>MTERIRNVALRSKVCPAETASELIKHGDVVGTSGFTGAGYPKEVPKALAQRMEAAHDRGEKYQISLITGASTGPQLDGELAKANGVYFRSPFNTDATMRNRINAGETEYFDNHLGQVAGRAVQGNYGKFNIALVEATAITEDGGIVPTSSVGNSQTFLNLAEKVIIEVNEWQNPMLEGIHDIWDGNVSGVPTRDIVPIVRADQRVGGPVLRVNPDKIAAIVRTNDRDRNAPFAAPDETAKAIAGYLLDFFGHEVKQNRLPPSLLPLQSGVGNVANAVLEGLKEGPFENLVGYSEVIQDGMLAMLDSGRMRIASASSFSLSPEAAEEINNRMDFFRSKIILRQQDVSNSPGIIRRLGCIAMNGMIEADIYGNVNSTRVMGSKMMNGIGGSGDFARSSYLSIFLSPSTAKGGKISAIVPMAAHVDHIMQDAQIFVT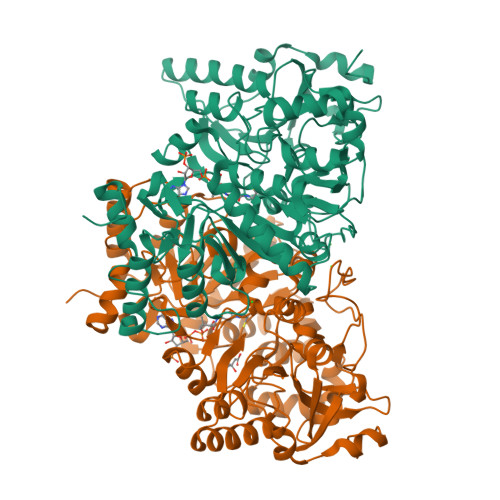EQGLADLRGLSPVQRAREIISKCAHPDYRPMLQDYFDRALKNSFGKHTPHLLTEALSWHQRFIDTGTMLPS[2x]>MEESQSKQESNTRVAQHGSQQDVDPTFQTKRALEKERSKPRPRPLPRVQLQSLPGWSSTSKDVPLSQLIREMDHESRRCIHRSKKKLDRSEHISQGTIPEIYEKRKETISHTQSMEQKYLFQNFTKLLLLQKCCPGGSEKLVRESWHPCVPEEGGHMIEIQDLFDPNLDTEKKPQLVIIEGAAGIGKSTLARQVKRAWDEGQLYRDRFQHVFFFSCRELAQCKQLSLAELIAQGQEVPTAPTRQILSRPEKLLFILDGIDEPAWVLEDQNPELCVHWSQAQPVHTLLGSLLGKSILPEASLMLTARTTALQKLVPSLGQPHRVEVLGFSEFERKDYFYKYFAKERNTIIDFNLIGSIPVLLTLCEVPWVCWLLCTCLEKQMQQGEVLSLTSQTTTALCLKYLSLTIPGQHLSTQLRTLCSLAAEGICQRRTLFSKSDLCKQGLAEDAIATFLKIGVLQRQPSSLSYSFAHLCLQEFFAAMSYILEDSEEAHGDMGNDRTVETLVERYGRQNLFEAPTVRFLLGLLNTREMREMENIFACKFPWETKLKLLQSIIGEPFCQPCHLGLFHCLYENQEEELLTETMLCFPLTASGPNHMEATVFQTNVKRLVIQTDMELMVVTFCITFSHVRSLRLKGKGQQEYKLTAPAMVLYRWTPISEASWKVLFSNLKCTRNLEELDLSGNPLSYSAVRSLCTALRQPGCRLKTLWLVDCGLTSRCCSFLASMLSAHSRLAELDLRLNDLGDNGVRQLCEGLRNPACNLSILRLDQASLSEQVITELRALETKNPKLFISSTWMSHMTMPTENTDGEESLTSSKQQQQQSGDKHMEPLGTDDDFWGPSGPVS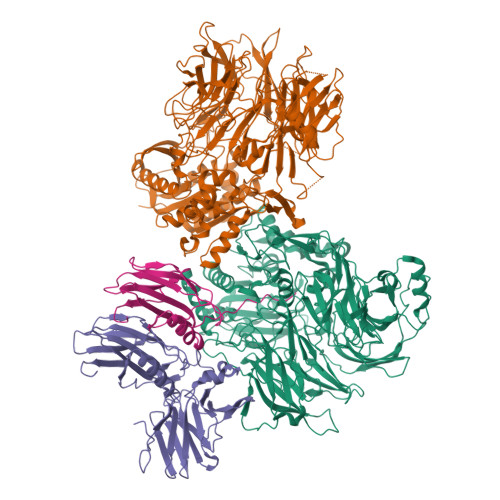TEVVDRERNLYRVRLPMAGSYHCPSTGLHFVVTRAVTIEIGFCAWSQFLHETPLQHSHMVAGPLFDIKAEHGAVTAVCLPHFVSLQEGKVDSSLFHVAHFQDHGMVLETPARVEPHFAVLENPSFSPMGVLLRMIPAVGHFIPITSITLIYYRLYLEDITFHLYLVPNDCTIRKAIDEEELKFQFVRINKPPPVDALYVGSRYIVSSSKEVEILPKELELCYRSPRESQLFSEIYVGNIGSGINLQLTDKKYMNLIWEALLKPGDLRPALPRMASAPKDAPALLHFVDQHREQLVARVTSVDPLLDKLHGLVLSEEDYETVRAEATNQDKMRKLFRGSRSWSWDCKDHFYQALKETHPHLIMDLLEKSGGVSVRL[2x];>MSGGVSPVEQVAAGDMDDTAARFCVQKHSWDGLRNIIHGSRKSSGLIVSKAPHDFQFVQKPDESGPHSHRLYYLGMPYGSRENSLLYSEIPKKVRKEALLLLSWKQMLDHFQATPHHGVYSREEELLRERKRLGVFGITSYDFHSESGLFLFQASNSLFHCRDGGKNGFMVSPMKPLEIKTQCSGPRMDPKICPADPAFFSFINNNDLWVANIETGEERRLTFCHQGSASVLDNPKSAGVATFVIQEEFDRFTGCWWCPTASWEGSGGLKTLRILYEEVDESEVEVIHVPSPALEERKTDSYRYPRTGSKNPKIALKLAELQTDHQGKIVSSCEKELVQPFSSLFPKVEYIARAGWTRDGRYAWAMFLDRPQQRLQLVLLPPALFIPTLESEAQWQEAARAIPKNVQPFIIYEEVTNVWINVHDIFHPFPQAEGQQDFCFLRANECKTGFCHLYRVTVDLKTNDYDWTEPLSPAEDEFKCPIKEEVALTSGEWEVLSRHGSKIWVNEQTKLVYFQGTKDTPLEHHLYVVSYESAGEIVRLTTPGFSHSCSMSQNFDMFVSHYSSVSTPPCVHVYKLSGPDDDPLHKQPRFWASMMEAASCPPDYVPPEIFHFHTRADVQLYGMIYKPHTLQPGRKHPTVLFVYGGPQVQLVNNSFKGIKYLRLNTLASLGYAVVVIDGRGSCQRGLHFEGALKNQMGQVEIEDQVEGLQYVAEKYGFIDLSRVAIHGWSYGGFLSLMGLIHKPQVFKVAIAGAPVTVWMAYDTGYTERYMDVPENNQQGYEAGSVALHVEKLPNEPNRLLILHGFLDENVHFFHTNFLVSQLIRAGKPYQLQIYPNERHSIRCRESGEHYEVTLLHFLQEHL[2x]> SPQREPQRVSHEQFRAALQLVVDPGDPRSYLDNFIKIGEGSTGIVCIATVRSSGKLVAVKKMDLRKQQRREL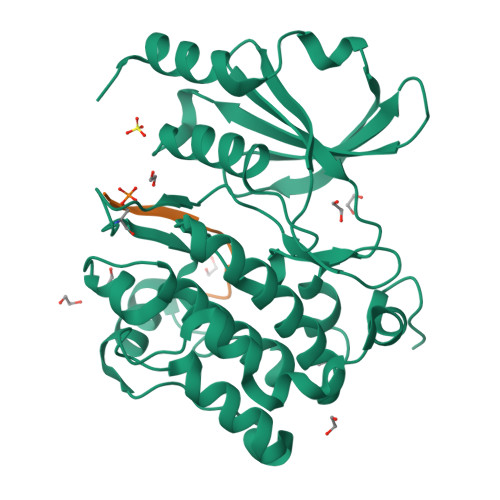LFNEVVIMRDYQHENVVEMYNSYLVGDELWVVMEFLEGGALTDIVTHTRMNEEQIAAVCLAVLQALSVLHAQGVIHRDIKSDSILLTHDGRVKLSDFGFCAQVSKEVPRRKSLVGTPYWMAPELISRLPYGPEVDIWSLGIMVIEMVDGEPPYFNEPPLKAMKMIRDNLPPRLKNLHKVSPSLKGFLDRLLVRDPAQRATAAELLKHPFLAKAGPPASIVPLMRQNRTR;> RRRRRSWYFDG> GPLGSMALVKKNQARNTQATDNKGASAYLNF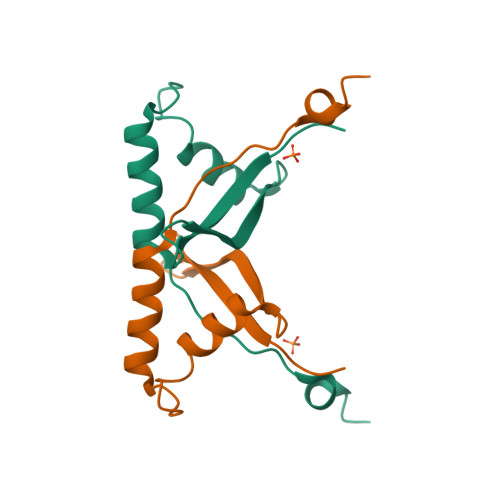HFPTRDGKDVRLVSLGLRADDALHMQLQEFLTVDDKGKPLSETAYAERCKKLVSRLIIKLGVTRSEEERALDL>MHHHHHHAAGIPMNNPAIKRIGNHITKSPEDKREYRGLELANGIKVLLISDPTTDKSSAALDVHIGSLSDPPNIAGLSHFLQHMLFLGTKKYPKENEYSQFLSEHAGSSNAFTSGEHTNYYFDVSHEHLEGALDRFAQFFLSPLFDESAKDREVNAVDSEHEKNVMNDAWRLFQLEKATGNPKHPFSKFGTGNKYTLETRPNQEGIDVRQELLKFHSAYYSSNLMAVVVLGRESLDDLTNLVVKLFSEVENKNVPLPEFPEHPFQEEHLKQLYKIVPIKDIRNLYVTFPIPDLQKYYKSNPGHYLGHLIGHEGPGSLLSELKSKGWVNTLVGGQKEGARGFMFFIINVDLTEEGLLHVEDIILHMFQYIQKLRAEGPQEWVFQELKDLNAVAFRFKDKERPRGYTSKIAGILHYYPLEEVLTAEYLLEEFRPDLIEMVLDKLRPENVRVAIVSKSFEGKTDRTEEWYGTQYKQEAIPDEVIKKWQNADLNGKFKLPTKNEFIPTNFEILPLEKEATPYPALIKDTAMSKLWFKQDDKFFLPKANLNFEFFSPFAYVDPLHSNMAYLYLELLKDSLNEYAYAAELAGLSYDLQNTIYGMYLSVKGYNDKQPILLKKIIEKMATFEIDEKRFEIIKEAYMRSLNNFRAEQPHQHAMYYLRLLMTEVAWTKDELKEALDDVTLPRLKAFIPQLLSRLHIEALLHGNITKQAALGIMQMVEDTLIE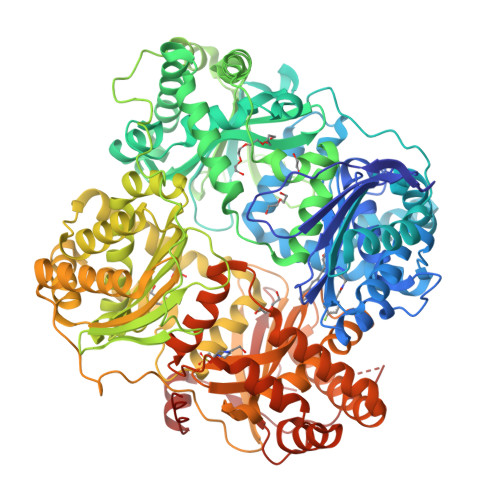HAHTKPLLPSQLVRYREVQLPDRGWFVYQQRNEVHNNSGIEIYYQTDMQSTSENMFLELFAQIISEPAFNTLRTKEQLGYIVFSGPRRANGIQGLRFIIQSEKPPHYLESRVEAFLITMEKSIEDMTEEAFQKHIQALAIRRLDKPKKLSAESAKYWGEIISQQYNFDRDNTEVAYLKTLTKEDIIKFYKEMLAVDAPRRHKVSVHVLAREMDSNPVVGEFPAQNDINLSQAPALPQPEVIQNMTEFKRGLPLFPLVKPHINFMAAKL[2x]> SNAMEELTLKGVTQYYAYVTERQKVHCLNTLFSRLQINQSIIFCNSSQRVELLAKKISQLGYSCFYIHAKMRQEHRNRVFHDFRNGLCRNLVCTDLFTRGIDIQAVNVVINFDFPKLAETYLHRIGRSGRFGHLGLAINLITYDDRFNLKSIEEQLGTEIKPIPSNIDKSLY;> GPLGSLKFESDFDFEKANEKFQEVLVDNLEKLNIEDKAEPEVEEKKDA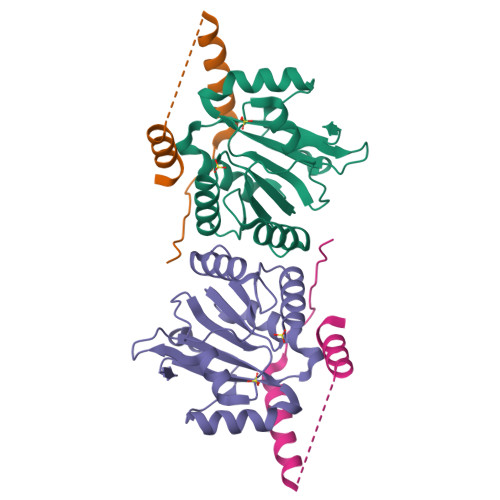AFYDKKTSFFDNISCESLEKAEGKTGRPDWKKERETNQETFG>TTIVSVRRNGHVVIAGDGQATLGNTVMKGNVKKVRRLYNDKVIAGFAGGTADAFTLFELFERKLEMHQGHLVKAAVELAKDWRTDRMLRKLEALLAVADETASLIITGNGDVVQPENDLIAIGSGGPYAQAAARALLENTELSAREIAEKALDIAGDICIYTNHFHTIEELSYKA[8x];>[4x]HHHHHHHSEMTPREIVSELDKHIIGQDNAKRSVAIALRNRWRRMQLNEELRHEVTPKNILMIGPTGVGKTEIARRLAKLANAPFIKVEATKFTEVGYVGKEVDSIIRDLTDAAVKMVRVQAIEKNRYRAEELAEERILDVLIPPAKNNWGQTEQQQEPS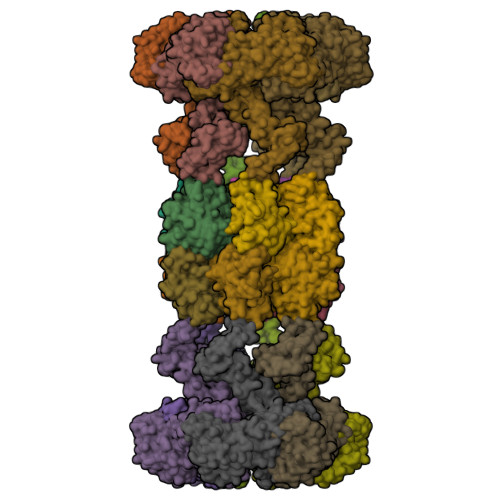AARQAFRKKLREGQLDDKEIEIDLAAAPMGVEIMAPPGMEEMTSQLQSMFQNLGGQKQKARKLKIKDAMKLLIEEEAAKLVNPEELKQDAIDAVEQHGIVFIDEIDKICKRGESSGPDVSREGVQRDLLPLVEGCTVSTKHGMVKTDHILFIASGAFQIAKPSDLIPELQGRLPIRVELQALTTSDFERILTEPNASITVQYKALMATEGVNIEFTDSGIKRIAEAAWQVNESTENIGARRLHTVLERLMEEISYDASDLSGQNITIDADYVSKHLDALVADEDLSRFIL(3M)-N~6~-(1,4-dimethyl-1H-pyrazol-3-yl)-3-(1-methyl-1H-imidazol-5-yl)-2,7-naphthyridine-1,6-diamine 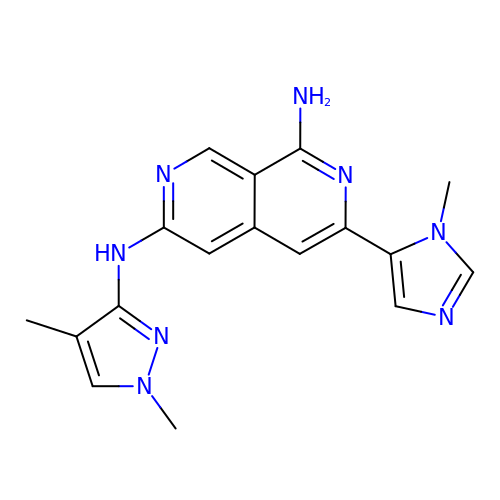| C17 H18 N8 | XPTAASNOZLTEFS-UHFFFAOYSA-N> MTALTEGAKLFEKEIPYITELEGDVEGMKFIIKGEGTGDATTGTIKAKYICTTGDLPVPWATILSSLSYGVFCFAKYPRHIADFFKSTQPDGYSQDRIISFDNDGQY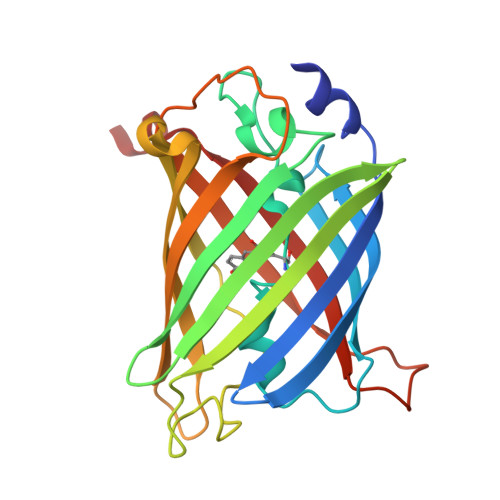DVKAKVTYENGTLYNRVTVKGTGFKSNGNILGMRVLYHSPPHAVYILPDRKNGGMKIEYNKAFDVMGGGHQMARHAQFNKPLGAWEEDYPLYHHLTVWTSFGKDPDDDETDHLTIVEVIKAVDLETYR4-[(6-CHLORO-2-NAPHTHALENYL)SULFONYL]-1-[[1-(4-PYRIDINYL)-4-PIPERIDINYL] METHYL]-2-PIPERAZINECARBOXYLIC ACID | C26 H29 Cl N4 O4 S | 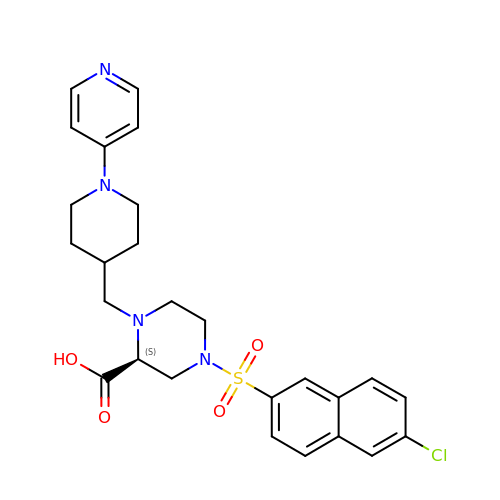QLUPDKQDBWRPGQ-VWLOTQADSA-N>[6x]GQQMMQYEWRKAELIGQLLNLGVTPGGVLLVHSSFRSVRPLEDGPLGLIEALRAALGPGGTLVMPSWSGLDDEPFDPATSPVTPDLGVVSDTFW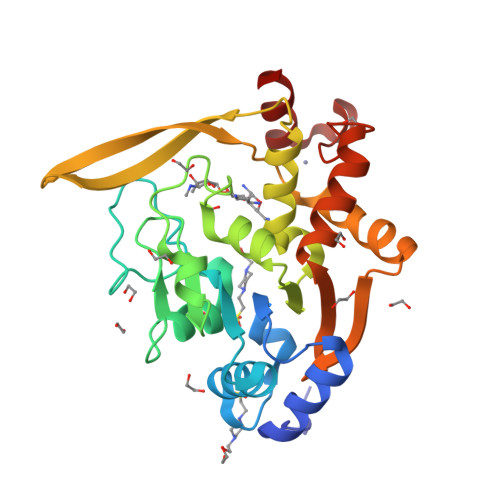RLPNVKRSAHPFAFAAAGPQAEQIISDPLPLPPHSPASPVARVHELDGQVLLLGVGHDANTTLALAELMAKVPYGVPRHCTILQDGKLVRVDYLENDHCCERFALADRWLKEKSLQKEGPVGHAFARLIRSRDIVATALGQLGRDPLIFLHPPEAGCEECDAARQSIG> MSTNKVNKERTFLAVKPDGVARGLVGEIIARYEKKGFVLVGLK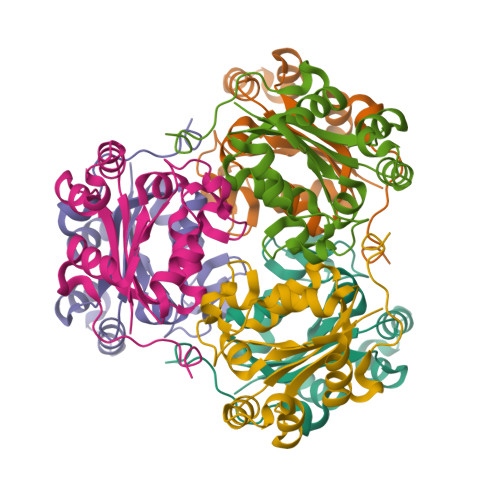QLVPTKDLAESHYAEHKERPFFGGLVSFITSGPVVAMVFEGKGVVASARLMIGVTNPLASAPGSIRGDFGVDVGRNIICGSDSVESANREIALWFKPEELLTEVKPNPNLYE> MEKKLPRIKALLTPGEVAKRSGVAVSALHFYESKGLITSIRNSGNQR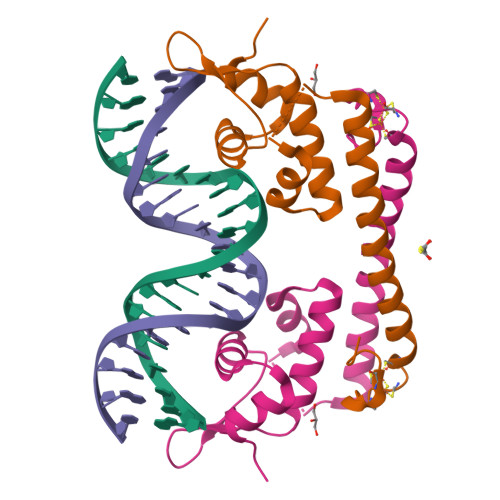RYKRDVLRYVAIIKIAQRIGIPLATIGEAFGVLPEGHTLSAKEWKQLSSQWREELDRRIHTLVALRDELDGCIGCGCLSRSDCPLRNPGDRLGEEGTGARLLEDEQN>[4x]SMGPTSQRRGSLQLWQFLVALLDDPSNSHF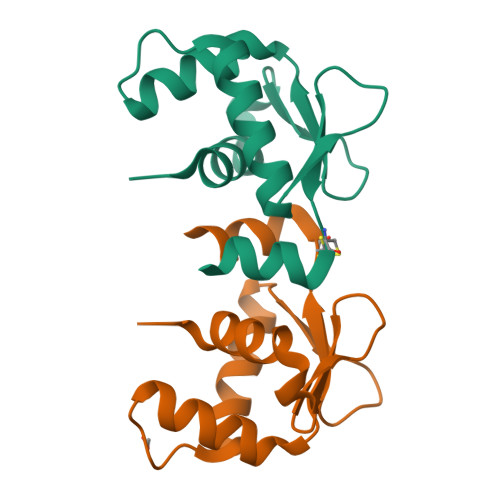IAWTGRGMEFKLIEPEEVARRWGIQKNRPAMNYDKLSRSLRYYYEKGIMQKVAGERYVYKFVCDPEALFSMAFSDN> MVLNKVTYKINAYKIKEEFIPKEVHFYRIKSFVNEAFNFYRFVNFYGGMIINKKDKSFVLPYKVDNKVLKYKDGNNEIPIDIEYIKSLKLEYVKPEIAEKLVRGYLKSVHKIEPELSRIIKNIRKHKVVENIKVESYCEYEVKKHDGDYYLILNFRHTASITKHLWDFVNRDKALLEEYVGKKIIFKPNPKVRYTISLVDAPNPQKIEEIMSHIIKYYKWSEDMVKSTFGEIDYNQPIMYCEEILEPFAPQFCNLVFYMDELDSYILKELQSYWRLSNENKGKIINEIAKKLRFIDNTPKELEFMKFNNTPLLVKDVNKNPTKIYSTNTLFTWIYNQNAKIYLPYDVPEIIRNKNLLTYILIDEEIKDELKAIKDKVNKMFRNYNKIANKTELPKFNYANRWKYFSTDDIRGIIKEIKSEFNDEICFALIIGKEKYKDNDYYEILKKQLFDLKIISQNILWENWRKDDKGYMTNNLLIQIMGKLGIKYFILDSKTPYDYIMGLDTGLGIFGNHRVGGCTVVYDSEGKIRRIQPIETPAPGERLHLPYVIEYLENKANIDMENKNILFLRDGFIQNSERNDLKEISKELNSNIEVISIRKNNKYKVFTSDY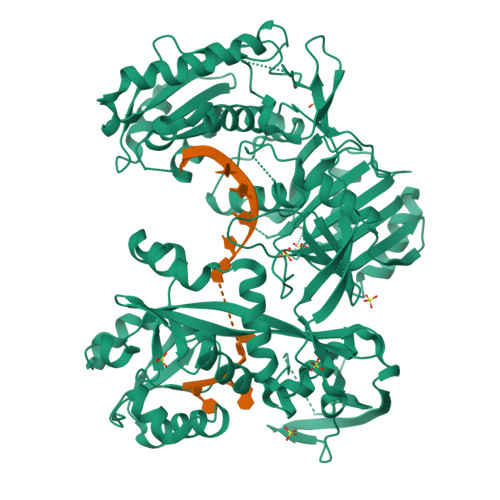RIGSVFGNDGIFLPHKTPFGSNPVKLSTWLRFNCGNEEGLKINESIMQLLYDLTKMNYSALYGEGRYLRIPAPIHYADKFVKALGKNWKIDEELLKHGFLYFI6-HYDROXY-1,6-DIHYDRO 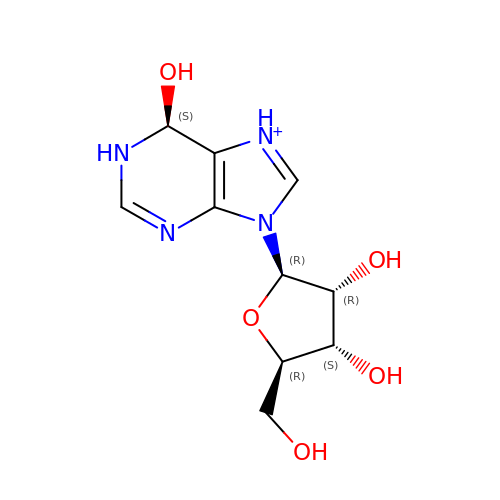PURINE NUCLEOSIDE | C10 H15 N4 O5 | WGRXVKRHIMUTPD-YOHZANMFSA-O> XQAD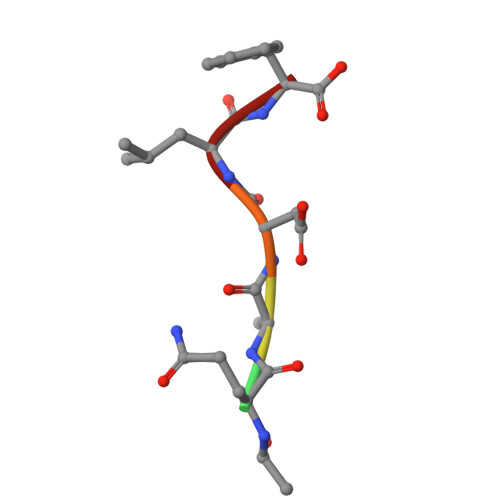LF> MQQASTPTIGMIVPPAAGLVPADGARLYPDLPFIASGLGLGSVTPEGYDAVIESVVDHARRLQKQGAAVVSLMCTSLSFYRG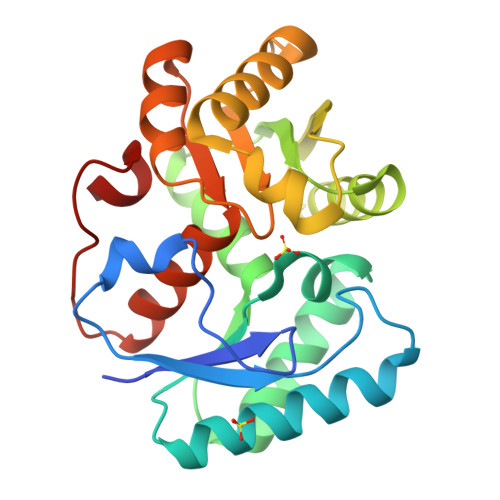AAFNAALTVAMREATGLPCTTMSTAVLNGLRALGVRRVALATAYIDDVNERLAAFLAEESLVPTGCRSLGITGVEAMARVDTATLVDLCVRAFEAAPDSDGILLSCGGLLTLDAIPEVERRLGVPVVSSSPAGFWDAVRLAGGGAKARPGYGRLFDES> HVPLTFDLPFEELLTYPGRTPRPADHDEYWDRGLADLAAVPADVVIEPAEFTTPLARCSHLWFTGTGGVRVHAKLLRPVAPVEPHPALLQFHGYTGNSGDWSSRLHYVALGYTVAALDCRGQAGLSVGEAPVENWSMASYLLRGIDDDAADNLALRHLFLDTARLAQ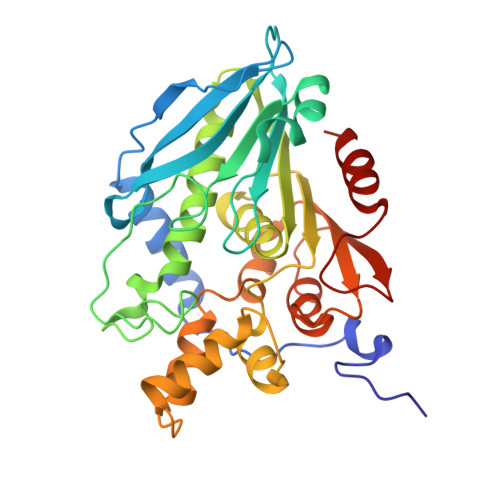IVLAMDDVDPDRVAATGYSQGGGLTLACAALEPRIRLAAPVYPFLCDFRRAWEMDLEKGPYNEITTYFRARDPRHLREEEIFSRLGYVDVQHLAPRVRAEVLMTVSLADKICPPSTQFAAYNKLGGPKDYRLYPDFAHETLPGTDDAIFTFLQGL> VVTYNTLIDGLAKAGRLEEALQLFQEMKEKGVKPDVVTYNTLID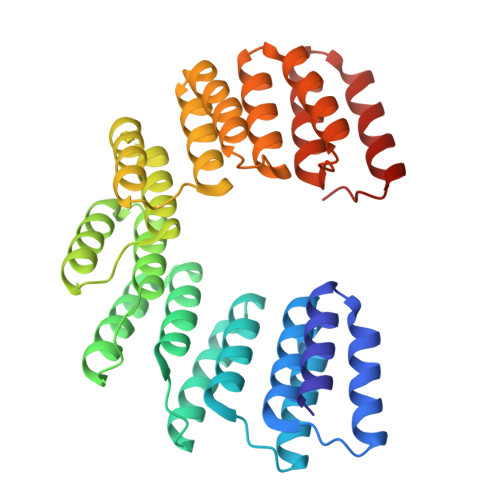GLAKAGRLEEALQLFQEMKEKGVKPDVVTYNTLIDGLAKAGRLEEALQLFQEMKEKGVKPDVVTYNTLIDGLAKAGRLEEALQLFQEMKEKGVKPDVVTYNTLIDGLAKAGRLEEALQLFEEMKEKGVKPDVVTYNTLIDGLAKAGRLEEALQLFQEMKEKGVKPDVVTYNTLIDGLAKAGRLEEALQLFEEMKEKGVKPDVVTYNTLIDGLAKAGRLEEALQLFEEMKEKGVKPDVVTYNTLIDGLAKAGRLEEALQLFQEMKEKGVKPD>MEEAYLALGKKILEEGHFKEDRTGTGTYSLFGYQMRFDLAKGFPLLTTKRVPFGLIKSELLWFLKGDTNIRYLLERNNHIWDEWAFERYVKSADYQGPDMTDFGHRVLQDPAFAEQYKEEHQKFCDAILNDAEFAEKYGELGNIYGAQWRHWETKDGSFIDQLANVIEMIKTNPDSRRLIVSAWNPEDVPSMALPPCHTMFQFYVNEGKLSCQLYQRSADVFLGVPFNIASYALLTHLIAHETGLEVGEFVHTLGDAHLYQNHVEQMQEQLSREVRSFPTLVLNPDKASVFDFDMEDIKVEGYDPHPTIKAPIAV[4x]

Thymidylate synthase (TS, EC 2.1.1.45) is a ubiquitous enzyme that catalyzes the reductive methylation of 2′-deoxyuridine-5′-monophosphate (dUMP) to 2′-deoxythymidyne-5′-monophosphate (dTMP) using N5,N10-methylenetetrahydrofolate (mTHF) as a cofactor. In cells, TS provides the only synthetic source of dTMP necessary for DNA biosynthesis. TS works as an obligate homodimer, having residues from both enzyme subunits that contribute to substrate binding in each catalytic site. TS subunits are characterized by two domains, known as large and small domains (LD and SD, respectively).

The structure of EfTS in complex with the substrate dUMP was determined to be 1.75 Å resolution. While subunits A and C where dUMP is bound display the open conformation, subunits B and D where 5-FTHF is bound are in the closed conformation. The cofactor-analogue (6S)-5-formyl-6-tetrahydrofolate (5-FTHF) is entrapped in the active sites of subunits B and D by the same tight network of interactions already observed in the substrate-free form of the enzyme. Moreover, in these subunits, the catalytic Cys197 is modified as S,S-(2-hydroxylethyl)thiocysteine (CME197) by the reaction with β-mercaptoethanol (added to the protein buffer during the purification process). In the partner subunits (A and C), the electron density of the catalytic Cys197 suggests that it had been oxidized to sulfenic acid (S-oxycysteine, CSX197 in Figure 3). Despite the oxidation of Cys197, the substrate dUMP populates the active site, showing its uracil moiety positioned just above the cysteine sulphur (C6–Sγ distance of ~3.7 Å). The dUMP phosphate is salt-bridged to Arg22, Arg217, Arg177’, and Arg178’ (the last two from the partner subunit) and it is further H-bonded to the hydroxyl of Ser218. The most evident rearrangement concerns the flexible loop 18–26, which moves towards the catalytic cavity in the dUMP-bound subunits, exposing Arg22 inside the phosphate recognition pocket. The movement of Arg22, whose Cα shifts by ~5.8 Å, is fundamental to create the four-arginine cluster that anchors the dUMP phosphate in the substrate site. Remarkably, despite the full occupancy of the substrate site by dUMP and the movement of the 18–26 loop towards dUMP, the SD retains the open conformation, in which it is widely unstructured. This observation strongly suggests that in EfTS, the open/closed transition occurs as a biphasic process in which the dUMP accommodation triggers the closure of the loop 18–26, whereas the binding of the cofactor (or analogue) induces the movement and the organization of the whole SD.> MLNQELELSLNMAFARAREHRHEFMTVEHLLLALLSNPSAREALEACSVDLVALRQELEAFIEQTTPVLPASEEERDTQPTLSFQRVLQRAVFHVQSSGRNEVTGANVLVAIFSEQESQAAYLLRKHEVSRLDVVNFISHGTRKDEPTQSSDPGSQPNSEEQAGGEERMENFTTNLNQLARVGGIDPLIGREKELERAIQVLCRRRKNNPLLVGESGVGKTAIAEGLAWRIVQGDVPEVMADCTIYSLDIGS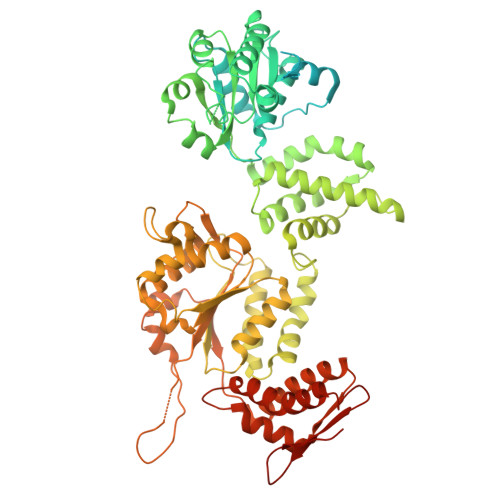LLAGTKYRGDFEKRFKALLKQLEQDTNSILFIDEIHTIIGAGAASGGQVDAANLIKPLLSSGKIRVIGSTTYQEFSNIFEKDRALARRFQKIDITEPSIEETVQIINGLKPKYEAHHDVRYTAKAVRAAVELAVKYINDRHLPDKAIDVIDEAGARARLMPVSKRKKTVNVADIESVVARIARIPEKSVSQSDRDTLKNLGDRLKMLVFGQDKAIEALTEAIKMARAGLGHEHKPVGSFLFAGPTGVGKTEVTVQLSKALGIELLRFDMSEYMERHTVSRLIGAPPGYVGFDQGGLLTDAVIKHPHAVLLLDEIEKAHPDVFNILLQVMDNGTLTDNNGRKADFRNVVLVMTTNAGVRETERKSIGLIHQDNSTDAMEEIKKIFTPEFRNRLDNIIWFDHLSTDVIHQVVDKFIVELQVQLDQKGVSLEVSQEARNWLAEKGYDRAMGARPMARVIQDNLKKPLANELLFGSLVDGGQVTVALDKEKNELTYGFQSAQKHKAEAAH>GIAGKEKSEEWAKYYPRQFDSWKKTKEYDSFTDMLAKDPALVIAWSGYAFSKDYNSPRGHYYALQDNVNSLRTGAPVDAKTGPLPTACWTCKSPDVPRLIEEDGELEYFTGKWAKYGSQIVNVIGCANCHDDKTAELKVRVPHLNRGLQAAGLKTFEESTHQDKRTLVCAQCHVEYYFKKTEWKDAKGADKTAMVVTLPWANGVGKDGNAGVEGMIKYYDEINFSDWTHNISKTPMLKAQHPGFEFWKSGIHGQKGVSCADCHMPYTQEGSVKYSDHQVKENPLDSMDQSCMNCHRESESKLRGIVHQKYERKEFLNKVAFDNIGKAHLETGKAIEAGASDEELKEVRKLIRHGQFKADMAIAAHGNYFHAPEETLRLLAAGSDDAQKARLLLVKILAKHGVMDYIAPDFDTKDKAQKLAKVDIAALAAEKM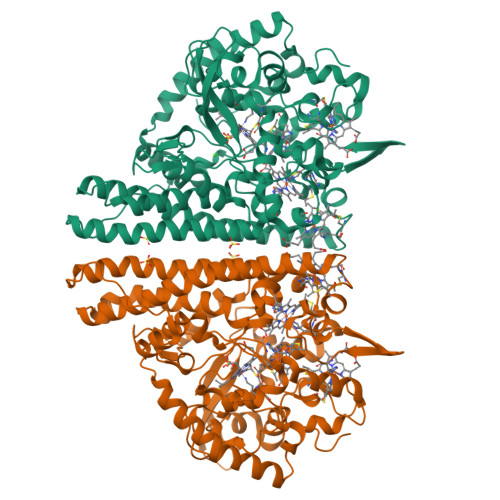KFKQTLEQEWKKEAKAKGRANPELYKDVDTINDGKSSWNKK[3x]>[7x]MANTDYAGNLTRPHWGGAASDVDIHLEVYQNEVDTRFQYQAMFLGLSSQRSVADRSNTYRIDRLNTSSVKGRTSGVALEPTPVRNDKMLIVVDTVLYIRNPIDYQDDWTA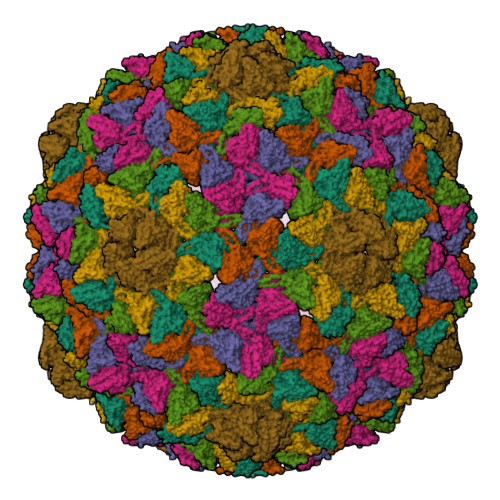PDFLTEMGQNNGSEFAEVFDQAHLIQLIKGRSWVAPAHLKPAFSDGIEIEATIDSDVTTQAGMEANAIAINQAHKAGIDELIKRKVPLNDMITLVSTEIYSLLLEHPKLFNKDWGDANANGYKERRAVLMNGIPVVECTEFPDAGTHPLGSAYTVTADDAKCRMVTFSKSRTLVTVEAKPFTSRIWDDEQNFANVLDCYAMYQVGERRPDTAAVVKFNEAP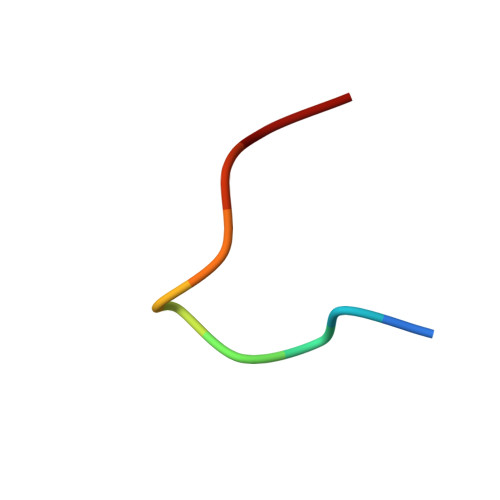> ACSSIWCPDG N-(5-{[(7-methyl-4-oxo-4H-pyrido[1,2-a]pyrimidin-2-yl)methyl]sulfanyl}-1,3,4-thiadiazol-2-yl)-N'-[3-(trifluoromethyl)phenyl]urea | C20 H15 F3 N6 O2 S2 | 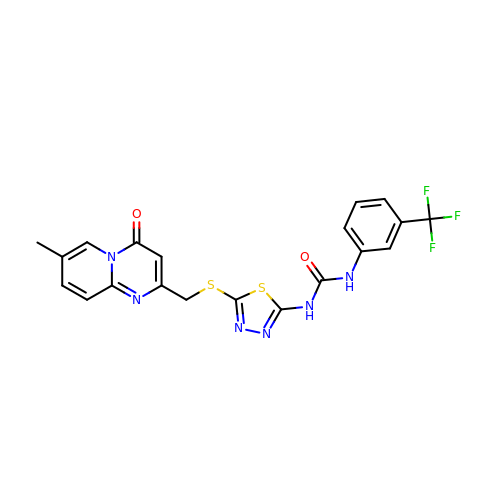OQDBRNRNKHKMSL-UHFFFAOYSA-N N,N-DIETHYL-2-[(2-THIENYLCARBONYL)AMINO]-4,5,6,7-TETRAHYDRO-1-BENZOTHIOPHENE-3-CARBOXAMIDE | C18 H22 N2 O2 S2 | 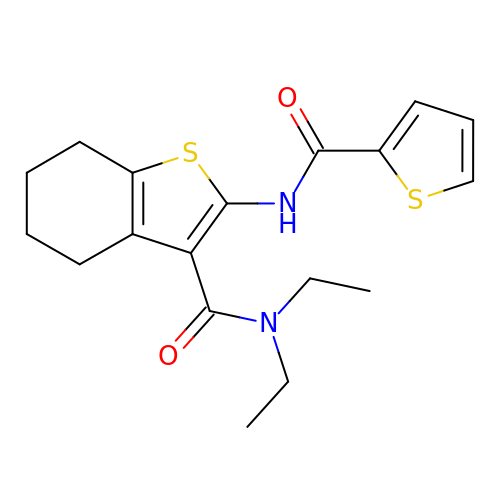NZTHBWHANVWSRX-UHFFFAOYSA-N>[6x]MKKIAFGCDHVGFILKHEIVAHL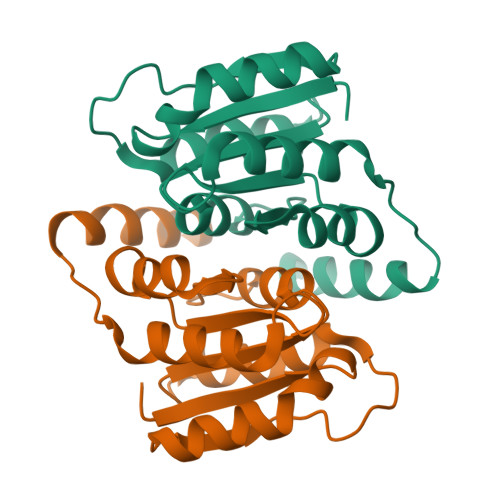VERGVEVIDKGTWSSERTDYPHYASQVALAVAGGEVDGGILICGTGVGISIAANKFAGIRAVVCSEPYSAQLSRQNNDTNVLAFGSRVVGLELAKMIVDAWLGAQYEGGRHQQRVEAITAIEQRRN>MSPSTNRKYPPLPVDKLEEEINRRMADDNKLFREEFNALPACPIQATCEAASKEENKEKNRYVNILPYDHSRVHLTPVEGVPDSDYINASFINGYQEKNKFIAAQGPKEETVNDFWRMIWEQNTATIVMVTNLKERKECKCAQYWPDQGCWTYGNIRVSVEDVTVLVDYTVRKFCIQQVGDMTNRKPQRLITQFHFTSWPDFGVPFTPIGMLKFLKKVKACNPQYAGAIVVHCSAGVGRTGTFVVIDAMLDMMHTERKVDVYGFVSRIRAQRCQMVQTDMQYVFIYQALLEHYLYGDTELEVTSLETHLQKIYNKIPGTSNNGLEEEFKKLTSIKIQNDKMRTGNLPANMKKNRVLQIIPYEFNRVIIPVKRGEENTDYVNASFIDGYRQKDSYIASQGPLLHTIEDFWRMIWEWKSCSIVMLTELEERGQEKCAQYWPSDGLVSYGDITVELKKEEECESYTVRDLLVTNTRENKSRQIRQFHFHGWPEVGIPSDGK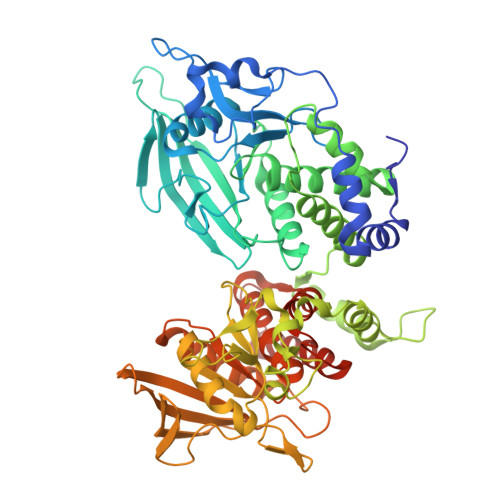GMISIIAAVQKQQQQSGNHPITVHCSAGAGRTGTFCALSTVLERVKAEGILDVFQTVKSLRLQRPHMVQTLEQYEFCYKVVQEYIDAFSDYANFKLEHHHHHH[2x]>GPGSPHKCKECGKAFHTPSQLSHHQKLHVGEKPYKCQECGKAFPSNAQLSLHHRVHTDEKCFECKECGKAFMRPSHLLR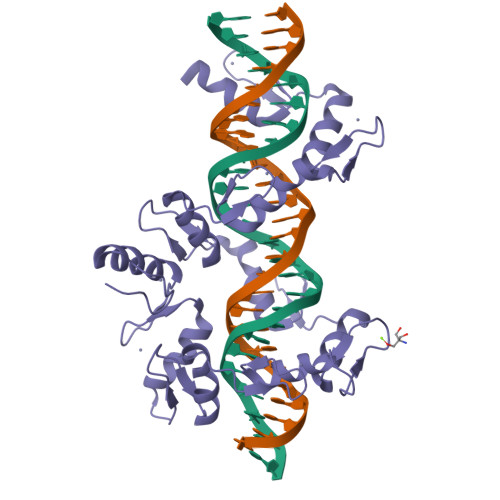HQRIHTGEKPHKCKECGKAFRYDTQLSLHLLTHAGARRFECKDCDKVYSCASQLALHQMSHTGEKPHKCKECGKGFISDSHLLRHQSVHTGETPYKCKECGKGFRRGSELARHQRAHSGDKPYKCKECGKSFTCTTELFRHQKVHTGDRPHKCKECGKAFIRRSELTHHERSHSGEKPYECKECGKTFGRGSELSRHQKIHTGEK[2x]6-CHLORO-2-(2'-FLUOROBIPHENYL-4-YL)-3-METHYLQUINOLINE-4-CARBOXYLIC ACID | C23 H15 Cl 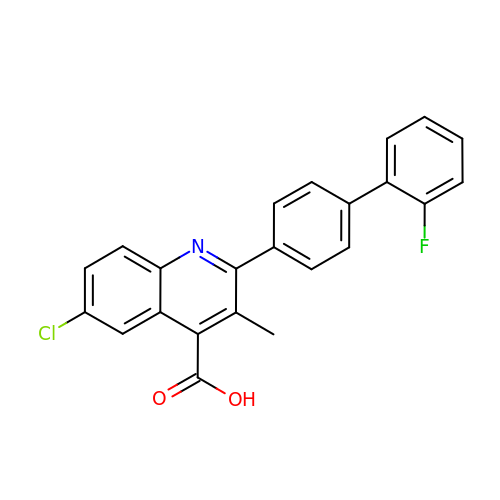F N O2 | JMFHBQIOFLEORU-UHFFFAOYSA-N G-quadruplexes (G4s) are highly stable nucleic acid secondary structures that can form in guanine-rich DNA or RNA1. G4 structures, in turn, comprise G-quartets stacked upon one another, stabilized by base stacking between the layers. Their stability can make G4s impediments to numerous cellular processes, including replication, transcription, and translation.

To better understand how G4 structures are resolved by helicases, the catalytic core domain of CsRecQ was crystallized in the presence of G4 DNA that included a 3′ single-stranded (ss) DNA loading site. Surprisingly, the 2.2 Å-resolution structure revealed a product complex of CsRecQ bound to unwound G4 DNA rather than a folded quadruplex. The RecQ/G4 product structure was very similar to the RecQ/duplex DNA structure, with a root mean square deviation of 0.68 Å among 511 Cα atoms. As was seen in the RecQ/duplex structure, the 3′ ssDNA is bound in an electropositive groove across the face of the helicase domain and it extends to dock in the ATP binding site of a symmetrically related molecule. Moreover, the helicase and winged-helix domains were closed around the unfolded G4. However, electron density was only observed for the three 3′-most guanines of the G4-forming DNA with the rest of the DNA apparently disordered within the crystal lattice. The 3′-most guanine base of the G4-forming sequence (G21), which is the first base within the folded G4 that would be encountered by the 3′–5′ translocating RecQ enzyme, was found sequestered in a guanine-specific pocket (GSP) on the surface of RecQ. The GSP forms hydrogen bonds with the guanine base using the sidechain hydroxyl and backbone amide of Ser245 and the sidechain carboxyl group from Asp312 of RecQ. These contacts are uniquely selective for guanine and, strikingly, they substitute for all of the hydrogen bonds that stabilize guanines within G4 structures. The GSP is capped on the 5ʹ end by the hydrophobic portion of the Lys248 sidechain and by Trp347 on the 3′ side.

> MGSSHHHHHHSSGLVPRGSHMAQAEVYSQETLAKQVLQETFGYQQFRPGQATIIDAVLEGRDCLVVMPTGGGKSLCYQIPALVKTGLTIVVSPLISLMKDQVDQLLANGVAAACLNSTQSREEQQAVLAGCRTGQVRLLYIAPERLMMDNFIDTLGYWDLAMVAVDEAHCISQWGHDFRPEYAALGQLRARFPAVPFMALTATADDTTRRDIVRLLGLDDPLIEISSFDRPNIRYMLMEKFKPLDQLMRYVQEQRGKSGIIYCNSRAKVEDTAARLQSRGISAAAYHAGLEHEVRASVQEKFQRDDLQIVVATVAFGMGINKPNVRFVVHFDIPRNIESYYQETGRAGRDGLPAEAMLFYDPADMAWLRRCLEEKAPGPLQDIERHKLNAMGAFAEAQTCRRLVLLNYFGEGRQAPCGNCDICLDPPRRYDGLVDAQKALSAIARVEQRFGMGYVVEVLRGANNQRIRELGHDKLKVYGIGRDQSQEHWVSVIRQLIHLGVVTQNIAQHSALQLTEAARPFLRGEAPLMLAVPRVAALKPR>MAEYTLPDLDWDYGALEPHISGQINELHHSKHHATYVKGANDAVAKLEEARAKEDHSAILLNEKNLAFNLAGHVNHTIWWKNLSPNGGDKPTGELAAAIADAFGSFDKFRAQFHAAATTVQGSGWAALGWDTLGNKLLIFQVYDQQTNFPLGIVPLLLLDMWEHAFYLQYKNVKVDFAK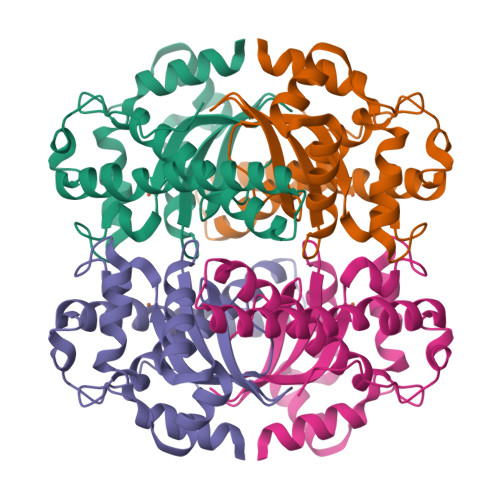AFWNVVNWADVQSRYAAATSQTKGLIFG[2x]>[2x]AIAENSSKEDYKIQSFDLETQKLLKTALKDPGSVDLEKVSSVIVDQSLKD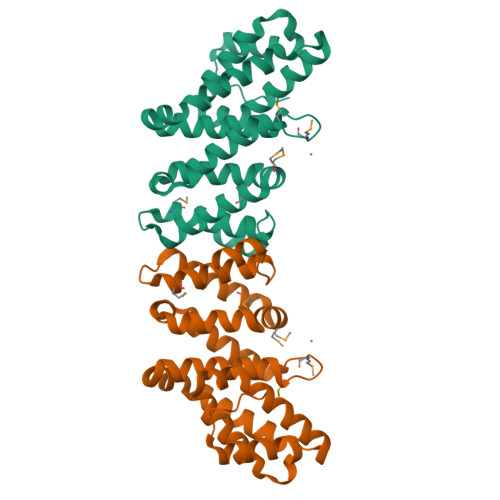QVFSREAGRICYTIVQAEAKQTNGSVFRRNLLNRLQQEFKAREETRKRSTQEWVCLVSFICNIFDYLKVNNMPMVALVHPVYDCLFRLAQSDALKNEEEVDCLVLQLHRIGDQLEKMNVQLMDELFNLLRDGFLLQEDLSSMGRLLLLEILEFRAGGWKLSDTAQKYYYSEVTD>[2x]MAGKKVLIVYAHQEPKSFNGSLKNVA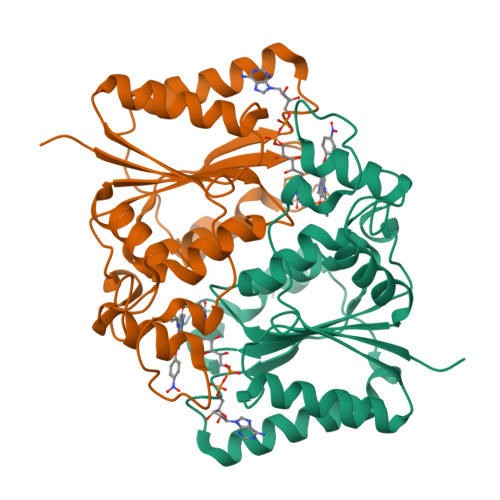VDELSRQGCTVTVSDLYAMNFEPRATDKDITGTLSNPEVFNYGVETHEAYKQRSLASDITDEQKKVREADLVIFQFPLYWFSVPAILKGWMDRVLCQGFAFDIPGFYDSGLLQGKLALLSVTTGGTAEMYTKTGVNGDSRYFLWPLQHGTLHFCGFKVLAPQISFAPEIASEEERKGMVAAWSQRLQTIWKEEPIPCTAHWHFGQHHHHHH>GSHMLGLIKKKANTLLGIDISSTSVKLLELSRSGGRYKVEAYAVEPLPPNAVVEKNIVELEGVGQALSRVLVKAKTNLKSAVVAVAGSAVITKTIEMEAGLSEDELENQLKIEADQYIPYPLEEVAIDFEVQGL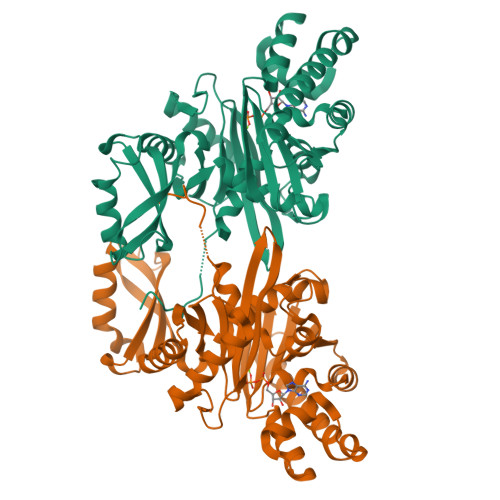SARNPERVDVLLAACRKENVEVREAALALAGLTAKVVDVEAYALERSYALLSSQLGADTDQLTVAVVDIGATMTTLSVLHNGRTIYTREQLFGGRQLTEEIQRRYGLSVEEAGLAKKQGGLPDDYDSEVLRPFKDAVVQQVSRSLQFFFAAGQFNDVDYIVLAGGTASIQDLDRLIQQKIGTPTLVANPFADMALNGKVNAGALASDAPALMIACGLALRSFD[2x]>MPSTDFADIPAAKKMKIDTCVLRFAKLTENALEPVRGSAKAAGVDLRSAYDVVVPARGKAIVKTDLQVQVPEGSYGRVAPRSGLAVKNFIDVGAGVVDEDYRG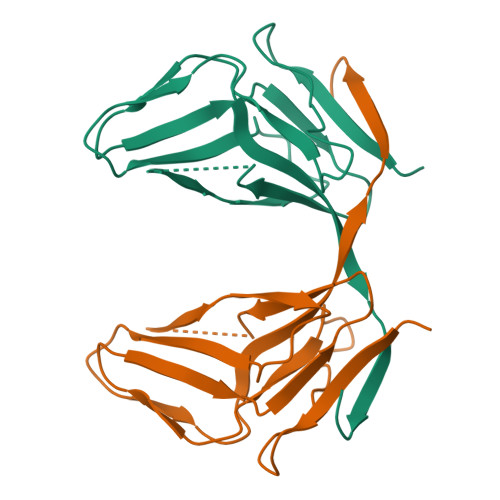NLGVVLFNHSDVDFEVKHGDRIAQFICERIFYPQLVMVDKLEDTERGEAGFGSTGVK[2x]>SMRKFGVV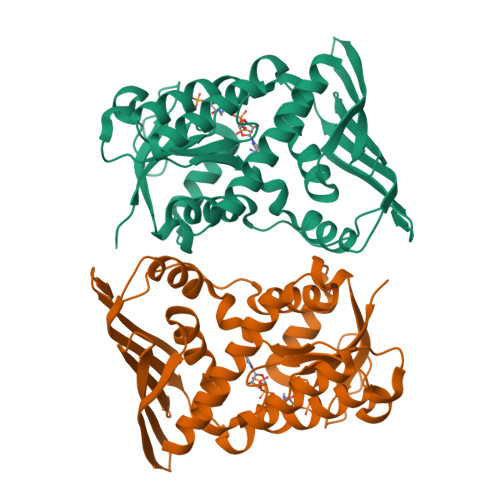VVGVGRAGSVRMRDLRNPHPSSAFLNLIGFVSRRELGSIDGVQQISLEDALSSQEVEVAYICSESSSHEDYIRQFLNAGKHVLVEYPMTLSLAAAQELWELAEQKGKVLHEEHVELLMEEFAFLKKEVVGKDLLKGSLLFTAGPLEEERFGFPAFSGISRLTWLVSLFGELSLVSATLEERKEDQYMKMTVCLETEKKSPLSWIEEKGPGLKRNRYLSFHFKSGSLENVPNVGVNKNIFLKDQNIFVQKLLGQFSEKELAAEKKRILHCLGLAEEIQKYCCSRK[4x]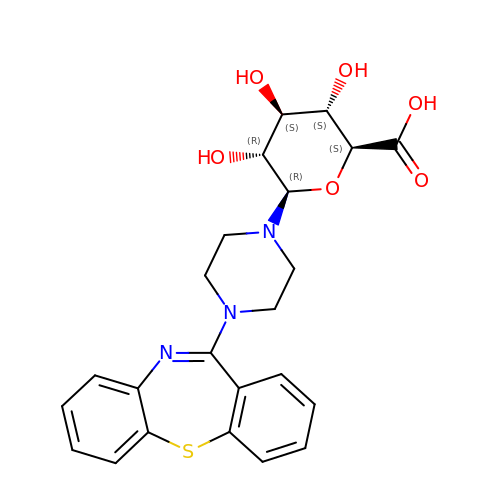11-(4-beta-D-glucopyranuronosylpiperazin-1-yl)dibenzo[b,f][1,4]thiazepine | C23 H25 N3 O6 S | UKCFGNFADWVWOZ-SXFAUFNYSA-N[(2R,3S,4R,5R)-4-(acetylamino)-3,5-dihydroxytetrahydrofuran-2-yl]methyl 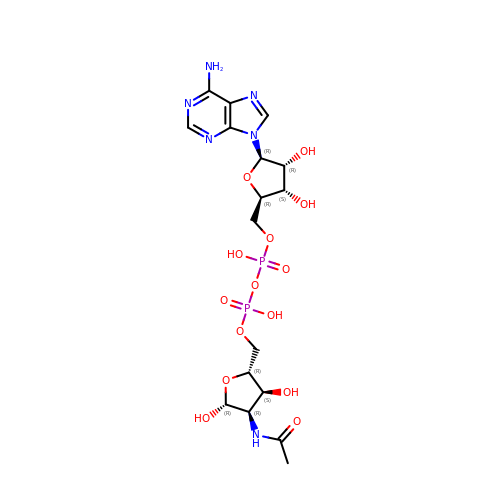[(2R,3S,4R,5R)-5-(6-amino-9H-purin-9-yl)-3,4-dihydroxytetrahydrofuran-2-yl]methyl dihydrogen diphosphate | C17 H26 N6 O14 P2 | YKUBGMLROVEQHG-YUGVQSHHSA-N>[4x]MPHVENASETYIPGRLDGKVALVTGSGRGIGAAVAVHLGRLGAKVVVNYANSTKDAEKVVSEIKALGSDAIAIKADIRQVPEIVKLFDQAVAHFGHLDIAVSNSGVVSFGHLKDV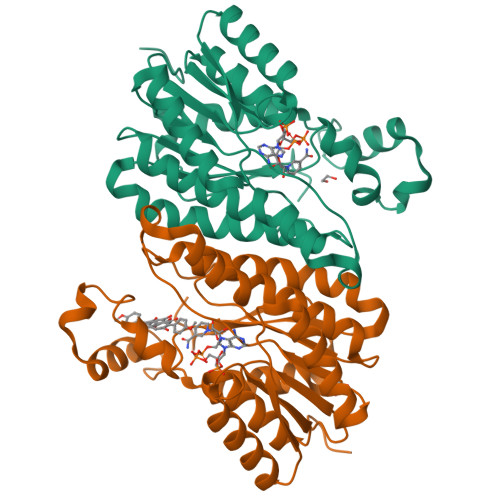TEEEFDRVFSLNTRGQFFVAREAYRHLTEGGRIVLTSSNTSKDFSVPKHSLYSGSKGAVDSFVRIFSKDCGDKKITVNAVAPGGTVTDMFHEVSHHYIPNGTSYTAEQRQQMAAHASPLHRNGWPQDVANVVGFLVSKEGEWVNGKVLTLDGGAA> GTPRVRTYTDVQKTGSVGRSIDVTSFKDYEELKSAIESMFGLEGLLTHPQSSGWKLVYVDYESDVLLVGDDPWEEFVGSVRSIRILSPTEVQQMSEEG;> GGPEAAAFVKVSMDGAPYLRKIDLRMYKSYDELSNALSNMFSSFTMGKHGGEEGMIDFMNERKLMDLVNSWDYVPSYENKDGNWMLVGDVPWPMFVD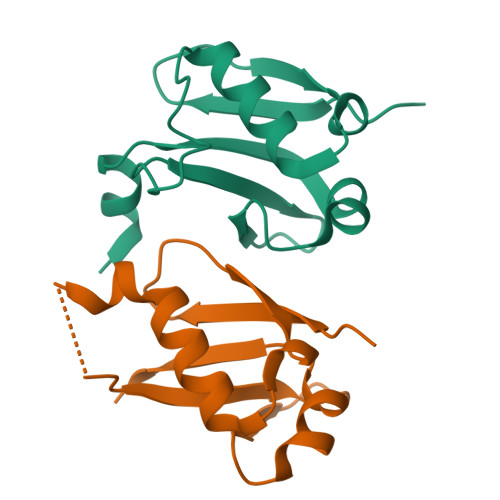TAKRLRLMKGSDAIGL>[2x]MGHHHHHHHHHHSSGENLYFQGHMNGRVQPRLMLGFLLILLVILALGSANMGALSLSFRTLWNTSTNDAMWHIWLNIRLPRVLLAVVVGCALAVSGTIMQGLFRNPLADPGLLGISSGAALCVGLIIVMPFSLPPLLALYSHMVGAFIGSLAISTIIFTLSRWGHGNLARLLLAGIAINALCGAAVGVLTYISDDQQLRQFSLWSMGSLGQAQWSTLLVASSLILPTCILGLLQARQLNLLQLGDEEAHYLGVNVRQAKLRLLLLSAILIGAAVAVSGVIGFIGLVVPHLIRMRIGADHRWLLPGAALGGACLLLTADTLARTLVAPAEMPVGLLTSLLGGPYFLWLILRQREQ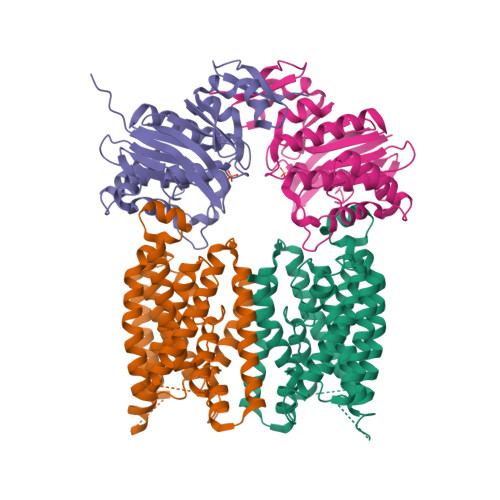RSG;>MVDMAVTPVALLEASHLHYHVQQQALINDVSLHIASGEMVAIIGPNGAGKSTLLRLLTGYLSPSHGECHLLGQNLNSWQPKALARTRAVMRQYSELAFPFSVSEVIQMGRAPYGGSQDRQALQQVMAQTDCLALAQRDYRVLSGGEQQRVQLARVLAQLWQPQPTPRWLFLDEPTSALDLYHQQHTLRLLRQLTRQEPLAVCCVLHDLNLAALYADRIMLLAQGKLVACGTPEEVLNAETLTQWYQADLGVSRHPESALPQIYLRQ[2x]> GSSPDKKWLGTPIEEMRRMPRCGIRLPLLRPSANHTVTIRVDLLRAGEVPKPFPTHYKDLWDNKHVKMPCSEQNLYPVEDENGERTAGSRWELIQTALLNKFTRPQNLKDAILKYNVAYSKKWDFTALIDFWDKVLEEAEAQHLYQSILPDMVKIALCLPNICTQPIPLLAAAMNHSITMSQEQIASLLANAFFCTFPRRNAKMKSEYSSYPDINFNRLFEGRSSRKPEKLKTLFCYFRRVTAAAPTGLVTFTRQSLEDFPEWERCEKPLTRLHVTYEGTIEENGQGMLQVDFANRFVGGGVTSAGLVQEEIRFLINPELIISRLFTEVLDHNECLIITGTEQYSEYTGYAETYRWSRSHEDGSERDDWQRRCTEIVAIDALHFRRYLDQFVPEKMRRELNKAYCGFLRPGVSSENLSAVATGNWGCGAFGGDARLKALIQILAAAAAERDVVYFTFGDSELMRDIYSMHIFLTERKLTVGDVYKLLLRYYNEECRNCSTPGPDIKLYPFIYHAVESCAETADHSGQRTGT

Protein ADP-ribosylation is a highly dynamic post-translational modification. The rapid turnover is achieved, among others, by ADP-(ribosyl)hydrolases (ARHs), an ancient family of enzymes that reverses this modification. Reversal of the bulk of PAR modification is mediated by poly(ADP-ribosyl)glycohydrolase (PARG) converting the polymer chain to a mono(ADP-ribosyl) (MAR) modification (Lin et al., 1997, Slade et al., 2011). For example, linkages to glutamate/aspartate are hydrolyzed by macrodomain proteins (Jankevicius et al., 2013, Rosenthal et al., 2013, Sharifi et al., 2013), whereas linkages to arginine and serine are cleaved by ARH1 and ARH3, respectively, two members of the structurally unrelated (ADP-ribosyl)hydrolases (ARHs) family (Fontana et al., 2017, Moss et al., 1988).

In order to probe whether the differences between the active sites have an effect on substrate recognition, we used the ADPr analogues adenosine diphosphate (hydroxymethyl)pyrrolidinediol (ADP-HPD) and -monoalcohol (ADP-HPM). These compounds were originally designed as PARG inhibitors and contain pyrrolidine instead of the distal ribose as well as differing in the number of hydroxyl substituents. The inability to coordinate MgII could account for the dramatic drop in Ki and IC50 observed for ARH3. This mode of inhibition stands in contrast to the structural studies on ADP-HPD as a PARG inhibitor (Kim et al., 2012, Lambrecht et al., 2015, Tucker et al., 2012). In PARG, the substrate is bound in a strained conformation due to the presence of a conserved phenylalanine (Phe875 in human PARG), which forces the distal ribose, in particular the linkage 1″ carbon, toward the catalytic loop. This conformation is further stabilized by extensive contacts between the Phe875 containing loop and the pyrophosphate moiety. The strained conformation, however, brings the ribose ring oxygen into the proximity of the Pα phosphate, which could stabilize the oxocarbenium reaction intermediate and explain the higher potency of ADP-HPD, which has a positively charged pyrrolidine nitrogen, in comparison with ADPr. In contrast, in PARG, the C6-linked amino group makes an electrostatic contact with Glu727 and water molecules. For example, PARG is being investigated as a chemotherapeutic target and promising inhibitors for it were recently discovered (Gravells et al., 2017, James et al., 2016), but the overlap in function between PARG and ARH3 remains to be elucidated. PARG activity appears to decrease with decreasing chain length and only low activity against oligomers of fewer than five units could be detected (Barkauskaite et al., 2013, Hatakeyama et al., 1986, Uchida et al., 1993).> MNLPTAQEVQGLMARYIELVDVGDIEAIVQMYADDATVENPFGQPPIHG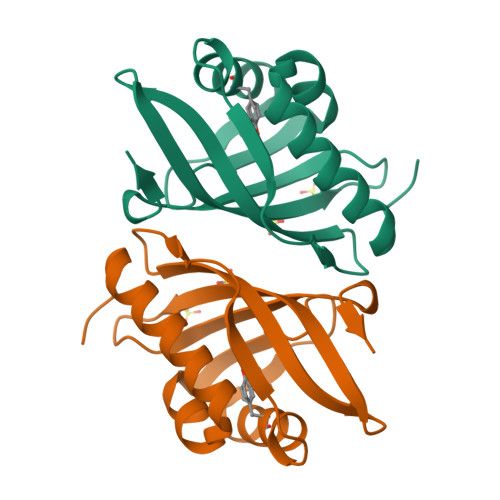REQIAAFXRQGLGGGKVRACLTGPVRASHNGCGAMPFRVEMVWNGQPCALDVIDVMRFDEHGRIQTMQAYWSEVNLSVREPQLVPR> MGSSHHHHHHSQDPMSNFIFGRYLPLDSVVHRLDPRAKLMLSFCYIIVVFLANNIWSYAILIAFTVGAILSSKISLGFFLKGIRPLLWLIVFTVVLQLLFSPAGGHTYFH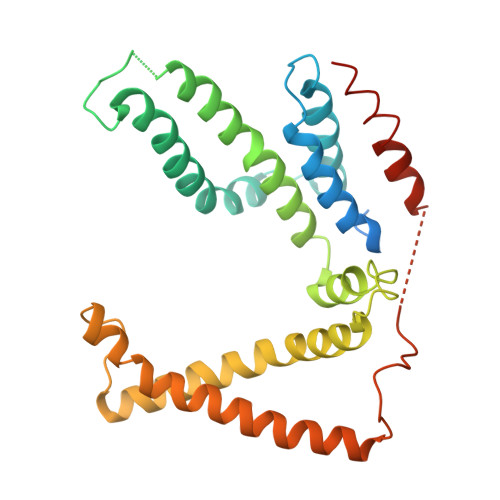WAFINVTQDGLINAGYIFVRFLLIIMMSTLLTLSTQPLDIATGLASLMKPLRWVKVPVDTLAMMLSIALRFVPTLMDEATKIMNAQRARGVDFGEGGLFKQAKSLIPLMVPLFMSAFNRAEDLSTAMEARGYQDSEHRSQYRILTWQRRDTVTWLLFLLGFVAILIFRHW> MASQPNSSAKKKEEKGKNIQVVVRCRPFNLAERKASAHSIVECDPVRKEVSVRTGGLADKSSRKTYTFDMVFGASTKQIDVYRSVVCPILDEVIMGYNCTIFAYGQTGTGKTFTMEGERSPNEEYTWEEDPLAGIIPRTLHQIFEKLTDNGTEFSVKVSLLEIYNEELFDLLNPSSDVSERLQMFDDPRNKRGVIIKGLEEITVHNKDEVYQILEKGAAKRTTAATLMNAYSSRSHSVFSV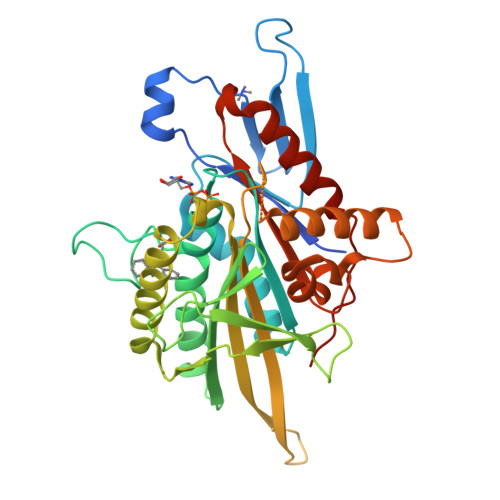TIHMKETTIDGEELVKIGKLNLVDLAGSENIGRSGAVDKRAREAGNINQSLLTLGRVITALVERTPHVPYRESKLTRILQDSLGGRTRTSIIATISPASLNLEETLSTLEYAHRAKNILNKPEVNQKL>[3x]MFKAIVSAATLRDALDSVSVLVDECKIRLNEESLSIRAVDPANVGMVDLTLDAAAFESYEAHGGVIGVNLSRLEEVAGMAG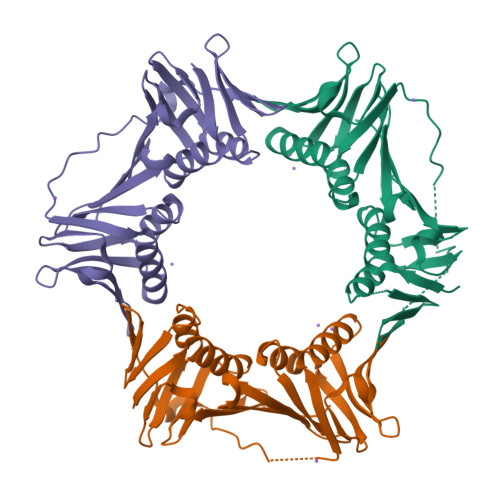AGDLIHLTLDEETRKLNIRIDGLSYTLALIDPDSIRQEPDIPDLDLAANIVLEGTHLDRGIKAADMVSDHIRLRVDGAEETFHIEAEGDTDDVDLSLPPADLISIEAGAADSLFSLDYLKDMNKAIPTDAEVTVELGEEFPVKLHYQIAEGMGTITYMLAPRIQSD>[12x]MERVAVVGVPMDLGANRRGVDMGPSALRYARLLEQLEDLGYTVEDLGD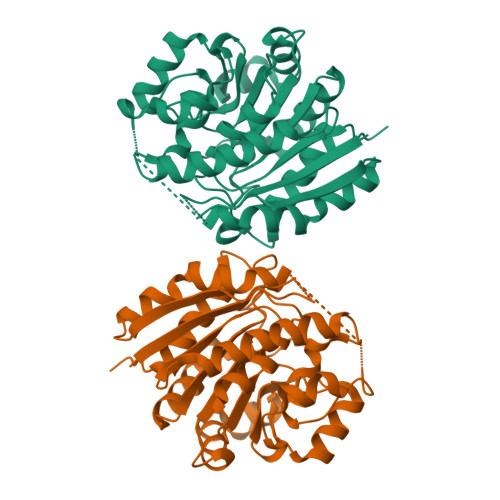VPVSLARASRRRGRGLAYLEEIRAAALVLKERLAALPEGVFPIVLGGDHSLSMGSVAGAARGRRVGVVWVDAHADFNTPETSPSGNVHGMPLAVLSGLGHPRLTEVFRAVDPKDVVLVGVRSLDPGEKRLLKEAGVRVYTMHEVDRLGVARIAEEVLKHLQGLPLHVSLDADVLDPTLAPGVGTPVPGGLTYREAHLLMEILAESGRVQSLDLVEVNPILDERNRTAEMLVGLALSLLGKRIF>MVTDSEKVAEYLRRATLDLRAARQRIRELESDPIAIVSMACRLPGGVNTPQRLWELLREGGETLSGFPTDRGWDLARLHHPDPDNPGTSYVDKGGFLDDAAGFDAEFFGVSPREAAAMDPQQRLLLETSWELVENAGIDPHSLRGTATGVFLGVAKFGYGEDTAAAEDVEGYSVTGVAPAVASGRISYTMGLEGPSISVDTACSSSLVALHLAVESLRKGESSMAVVGGAAVMATPGVFVDFSRQRALAADGRSKAFGAGADGFGFSEGVTLVLLERLSEARRNGHEVLAVVRGSALNQDGASNGLSAPSGPAQRRVIRQALESCGLEPGDVDAVEAHGTGTALGDPIEANALLDTYGRDRDADRPLWLGSVKSNIGHTQAAAGVTGLLKVVLALRNGELPATLHVEEPTPHVDWSSGGVALLAGNQPWRRGERTRRAAVSAFGISGTNAHVIVEEAPEREHRETTAHDGRPVPLVVSARSTAALRAQAAQIAELLERPDADLAGVGLGLATTRARHEHRAAVVASTREEAVRGLREIAAGAATADAVVEGVTEVDGRNVVFLFPGQGSQWAGMGAELLSSSPVFAGKIRACDESMAPMQDWKVSDVLRQAPGAP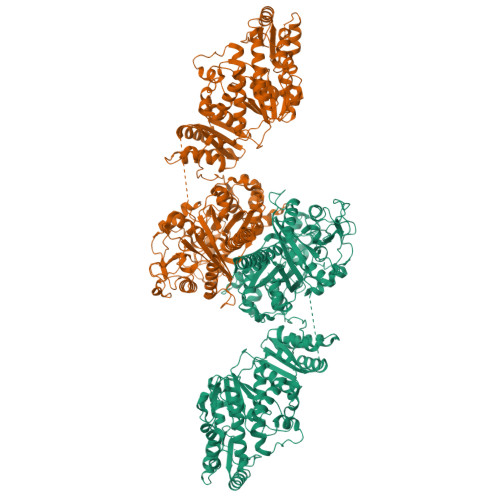GLDRVDVVQPVLFAVMVSLAELWRSYGVEPAAVVGHSQGEIAAAHVAGALTLEDAAKLVVGRSRLMRSLSGEGGMAAVALGEAAVRERLRPWQDRLSVAAVNGPRSVVVSGEPGALRAFSEDCAAEGIRVRDIDVDYASHSPQIERVREELLETTGDIAPRPARVTFHSTVESRSMDGTELDARYWYRNLRETVRFADAVTRLAESGYDAFIEVSPHPVVVQAVEEAVEEADGAEDAVVVGSLHRDGGDLSAFLRSMATAHVSGVDIRWDVALPGAAPFALPTYPFQRKRYWLQPAAPAAASDELAYRSSSVDKLAAALEHHHHHH[2x]>[2x]MASAGDVTRAALPRAQPRAEGPACVLGIGTAVPPAEFLQSEYPDFFFNITN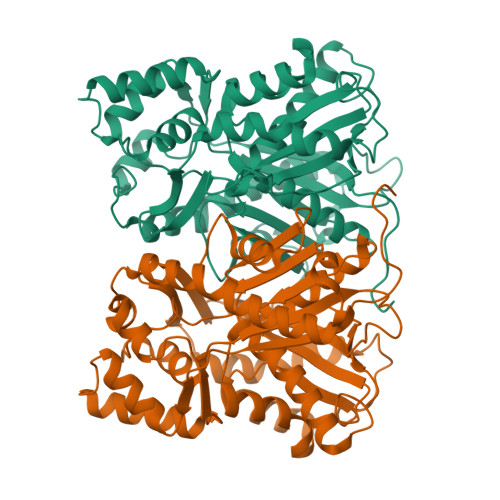CGEKEALKAKFKRICDKSGIRKRHMFLTEEVLKANPGICTYMEPSLNVRHDIVVVQVPKLAAEAAQKAIKEWGGRKSDITHIVFATTSGVNMPGADHALAKLLGLKPTVKRVMMYQTGCFGGASVLRVAKDLAENNKGARVLAVASEVTAVTYRAPSENHLDGLVGSALFGDGAGVYVVGSDPKPEVEKPLFEVHWAGETILPESDGAIDGHLTEAGLIFHLMKDVPGLISKNIEKFLNEARKPVGSPAWNEMFWAVHPGGPAILDQVEAKLKLTKDKMQGSRDILSEFGNMSSASVLFVLDQIRHRSVKMGASTLGEGSEFGFFIGFGPGLTLEVLVLRAAPNSA>MYIGIDLGTSGVKVILLNEQGEVVAAQTEKLTVSRPHPLWSEQDPEQWWQATDRAMKALGDQHSLQDVKALGIAGQMHGATLLDAQQRVLRPAILWNDGRCAQECTLLEARVPQSRVITGNLMMPGFTAPKLLWVQRHEPEIFRQIDKVLLPKDYLRLRMTGEFASDMSDAAGTMWLDVAKRDWSDVMLQACDLSRDQMPALYEGSEITGALLPEVAKAWGMATVPVVAGGGDNAAGAVGVGMVDANQAMLSLGTSGVYFAVSEGFLSKPESAVHSFCHALPQRWHLMSVMLSAASCLDWAAKLTGLSNVPALIAAAQQADESAEPVWFLPYLSGERTPHNNPQAKGVFFGLTHQHGPNELARAVLEGVGYALADGMDVVHACGIKPQSVTLIGGGARSEYWRQMLADISGQQLDYRTGGDVGPALGAARLAQIAANPEKSLIELLPQLPL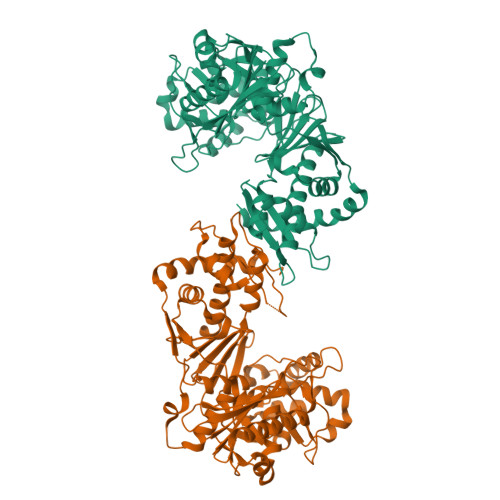EQSHLPDAQRYAAYQPRRETFRRLYQQLLPLMA[2x]>MLPLAALNMRVRRRLSLFLNVRTQVAADWTALAEEMDFEYLEIRQLETQADPTGRLLDAWQGRPGASVGRLLELLTKLGRDDVLLELGPSIEEDCQKYIAAALEHHHHHH[6x];>[4x]MGPITPSTYVRCLNVGLIRKLSDFIDPQEGWKKLAVAIKKPSGDDRYNQFHIRRFEALLQTGKSPTSELLFDWGTTNCTVGDLVDLLIQNEFFAPASLLLPDAVPLEHHHHHH;>[4x]ACYIYQLPSWVLDDLCRNMDALSEWDWMEFASYVITDLTQLRKIKSMEWVQGVSITR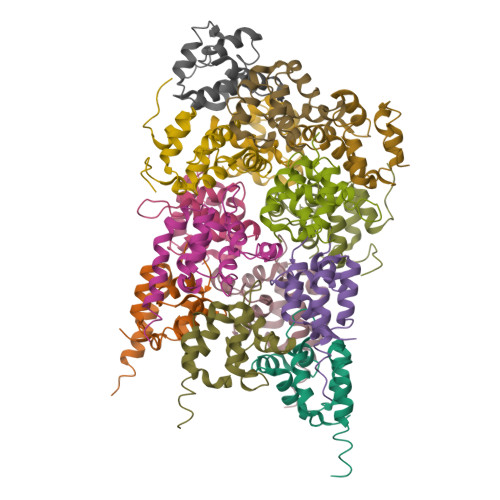ELLWWWGMRQATVQQLVDLLCRLELYRAAQIILNWKPAPEIRCPIPAFPDSVKP>[2x]MSEDKGPACYQVSDEQA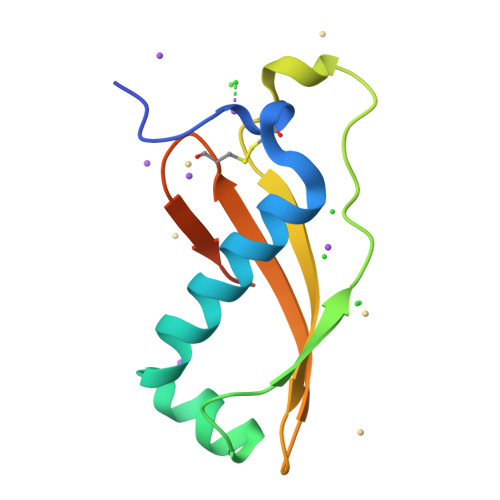RTFVKNDYLQRMKRWDNDVQLLGTEIPKITWEKIERSLTDVEDEKTLLVPFKAEGPDGKRMYYGMYHCEEGYVEYANDRSHHHHHH>[2x]MLPKLVITHRVHEEILQLLAPHCELITNQTDSTLTREEILRRCRDAQAMMAFMPDRVDADFLQACPELRVIGCALKGFDNFDVDACTARGVWLTFVPDLLTVPTAELAIGLAVGLGRHLRAADAFVRSGQFRGWQPRFYGTGLDNATVGFLGMGAIGLAMADRLQGWGATLQYHA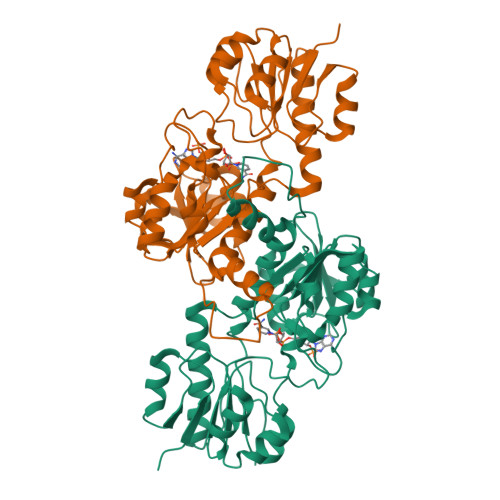RKALDTQTEQRLGLRQVACSELFASSDFILLALPLNADTLHLVNAELLALVRPGALLVNPCRGSVVDEAAVLAALERGQLGGYAADVFEMEDWARADRPQQIDPALLAHPNTLFTPHIGSAVRAVRLEIERCAAQNILQALAGERPINAVNRLP> MLADENDNHPLFTEGTYQAEVMENSPAGTPLTVLNGPILALDADEDVYAVVTYQLLGTHSDLFVIDNSTGVVTVRSGIIIDREAFSPPFLELLLLAEDIGQLNGTAHLFITILDDNDNWPTFSPPTYTVHLLENCPPGFPVLQVTATDEDSGLNGELVYRIEAGAQDRFLIHPVTGVIRVGNATIDREEQESYRLTVVAT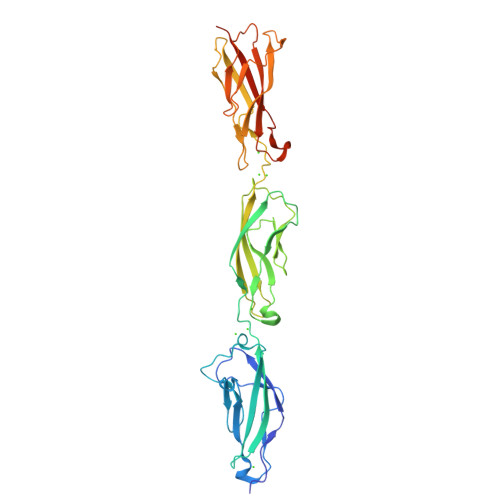DRGTVPLSGTAIVTILIDDINDSRPEFLNPIQTVSVLESAEPGTIIANVTAIDLDLNPKLEYHIISIVAKDDTDRLVPDQEDAFAVNINTGSVMVKSPLNRELVATYEVTLSVIDNASDLPEHSVSVPNAKLTVNILDVNDNLEHHHHHH A single ER‐localised Fic protein, FICD (HYPE), catalyses both AMPylation and deAMPylation of BiP. FICD is a class II Fic protein (with its αinh N‐terminal to its Fic domain) and an ER‐localised type II, single‐pass transmembrane protein, with a short cytoplasmic portion and a large luminal‐facing catalytic domain (Worby et al, 2009; Bunney et al, 2014). We report on the transition of FICD from a dimeric enzyme, that deAMPylates BiP, to a monomer with potent AMPylation activity. Mechanistically, monomerisation relieves a repressive effect allosterically propagated from the dimer interface to the inhibitory Glu234, thereby permitting AMPylation‐competent binding of MgATP.

Dimeric wild‐type FICD binds ATP (without magnesium) in an AMPylation‐incompetent mode. (i) The wild‐type dimer FICD structure displays a lack of density corresponding to a Mg2+ ion. As noted in other Fic AMPylases, this Mg2+ was coordinated by the α‐ and β‐phosphates of ATP/AMPPNP and Asp367 of the Fic motif (Xiao et al, 2010; Bunney et al, 2014; Khater & Mohanty, 2015b). Interestingly, in the dimeric wild‐type FICD:ATP structure, crystallised in the presence of MgATP, there was no density that could be attributed to Mg2+ (Fig 5B(i)). The only possible candidate for Mg2+ in this structure was a water density, located between all three phosphates, that fell in the Fic motif's anion hole—a position incompatible with Mg2+ coordination (Zheng et al, 2017). As previously observed in other ATP‐bound Fic proteins that possess an inhibitory glutamate, the nucleotide in FICD:ATP was in an AMPylation non‐competent conformation (Engel et al, 2012; Goepfert et al, 2013) that is unable to coordinate Mg2+: an essential cation for FICD‐mediated AMPylation (Ham et al, 2014). Moreover, the position of the ATP α‐phosphate precludes in‐line nucleophilic attack (by the hydroxyl group of BiP's Thr518) due to the proximity of the Fic domain flap residue Val316 (Figs 5C and EV4D). (i) The mode of ATP binding in wild‐type dimeric FICD sterically occludes the nucleophilic attack required for AMPylation. Note, His363 of FICD:ATP is in a non‐optimal flip state to facilitate general base catalysis. By contrast, dimeric wild‐type FICD is never able to bind MgATP competently, either in solution or in crystallo, due to its unperturbed allosteric dimer relay and consequently inflexible Glu234.

>[2x]SLEARAALNQALEMKRQGKREKAQKLFMHALKMDPDFVDALTEFGIFSEEDKDIIQADYLYTRALTISPYHEKALVNRDRTLPLVEEIDQRYFSIIDSKVKKVMSIPKGNSALRRVMEETYYHHIYHTVAIEGNTLTLSEIRHILETRYAVPGKSLEEQNEVIGMHAAMKYINTTLVSRIGSVTISDVLEIHRRVLGYVDPVEAGRFRTTQVLVGHHIPPHPQDVEKQMQEFVQWLNSEEAMNLHPVEFAALAHYKLVYIHPFIDGNGRTSRLLMNLILMQAGYPPITIRKEQRSDYYHVLEAANEGDVRPFIRFIAKCTETTLDTLLFATTEYSVALPEAQP> MANKAVNDFILAMNYDKKKLLTHQGESIENRFIKEGNQLPDEFVVIERKKRSLSTNTSDISVTATNDSRLYPGALLVVDETLLENNPTLLAVDRAPMTYSIDLPGLASSDSFLQVEDPSNSSVRGAVNDLLAKWHQDYGQVNNVPARMQYEKITAHSMEQLKVKFGSDFEKTGNSLDIDFNSVHSGEKQIQIVNFKQIYYTVSVDAVKNPGDVFQDTVTVEDLKQRGISAERPLVYISSVAYGRQVYLKLETTSKSDEVEAAFEALIKGVKVAPQTEWKQILDNTEVKAVILGGDPSSGARVVTGKVDMVEDLIQEGSRFTADHPGLP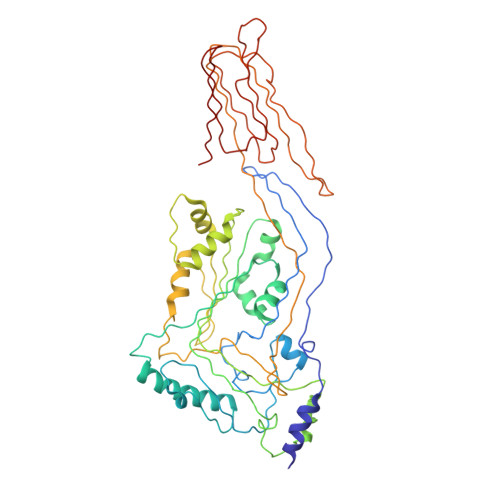ISYTTSFLRDNVVATFQNSTDYVETKVTAYRNGDLLLDHSGAYVAQYYITWDELSYNHQGKEVLTPKAWDRNGQDLTAHFTTSIPLKGNVRNLSVKIREATGLAWEWWRTVYEKTDLPLVRKRTISIWGTTLYPQVEDKVEND>GAMGSRADPRNQRVLLDEYSRQRGQITAGGQLLAYSVATDGRFRFLRVYPNPEVYAPVTGFYSLRYSSTALERAEDPILNGSDRRLFGRRLADFFTGRDPRGGNVDTTINPRIQQAGWDAMQQGCYGPCKGAVVALEPSTGKILALVSSPSYDPNLLASHNPEVQAQAWQRLGDNPASPLTNRAISETYPPGSTFKVITTAAALAAGATETEQLTAAPTIPLPGSTAQLENYGGAPCGDEPTVSLREAFVKSCNTAFVQLGIRTGADALRSMARAFGLDSPPRPTPLQVAESTVGPIPDSAALGMTSIGQKDVALTPLANAEIAATIANGGITM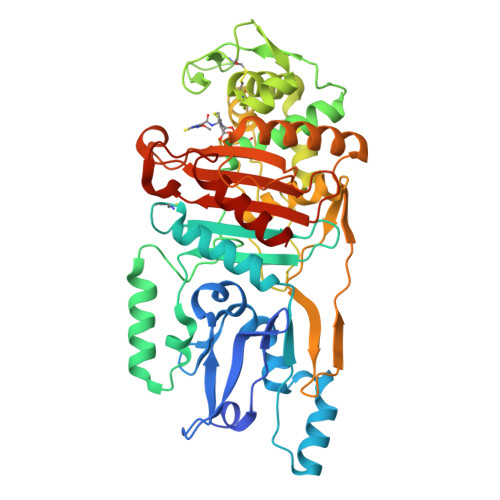RPYLVGSLKGPDLANISTTVRYQQRRAVSPQVAAKLTELMVGAEKVAQQKGAIPGVQIASKTGTAEHGTDPRHTPPHAWYIAFAPAQAPKVAVAVLVENGADRLSATGGALAAPIGRAVIEAALQGEP[2x]>SMGEAICSALPTIPYHKLA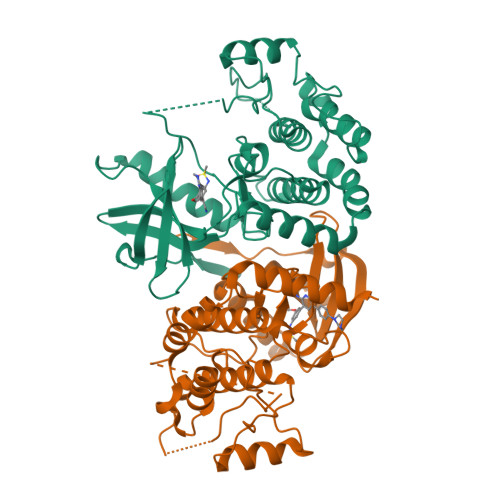DLRYLSRGASGTVSSARHADWRVQVAVKHLHIHTPLLDSERKDVLREAEILHKARFSYILPILGICNEPEFLGIVTEYMPNGSLNELLHRKTEYPDVAWPLRFRILHEIALGVNYLHNMTPPLLHHDLKTQNILLDNEFHVKIADFGLSKWRMMSLSQSRSSKSAPEGGTIIYMPPENYEPGQKSRASIKHDIYSYAVITWEVLSRKQPFEDVTNPLQIMYSVSQGHRPVINEESLPYDIPHRARMISLIESGWAQNPDERPSFLKCLIELEPVLRTFEEITFLEAVIQLKKTKLQSV[4x]>[4x]DYKDDDDKLHSQANLMRLKSDLFNRSPMYPGPTKDDPLTVTLGFTLQDIVKADSSTNEVDLVYYEQQRWKLNSLMWDPNEYGNITDFRTSAADIWTPDITAYSSTRPVQVLSPQIAVVTHDGSVMFIPAQRLSFMCDPTGVDSEEGATCAVKFGSWVYSGFEIDLKTDTDQVDLSSYYASSKYEILSATQTRQVQHYSCCPEPYIDVNLVVKFRERRAGNGFFRNLF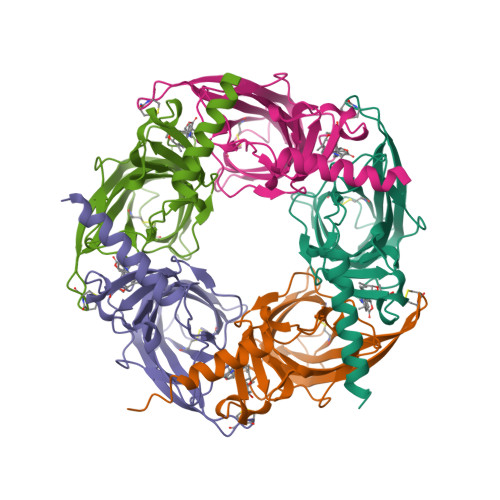D;> DYKDDDDLHSQANLMRLKSDLFNRSPMYPGPTKDDPLTVTLGFTLQDIVKADSSTNEVDLVYYEQQRWKLNSLMWDPNEYGNITDFRTSAADIWTPDITAYSSTRPVQVLSPQIAVVTHDGSVMFIPAQRLSFMCDPTGVDSEEGATCAVKFGSWVYSGFEIDLKTDTDQVDLSSYYASSKYEILSATQTRQVQHYSCCPEPYIDVNLVVKFRERRAGNGFFRNLFD> GQTKNEVSQDTIKTFTLPAIPQIMVAPEQRAEFLVKHYWDNVNFADTNYIHHPEITEQAWVDYCDILNHVPLKTAQEAIRKTIDRTNVDKKVFAYITDLADKYLYDPNSPMRNEEFYIPVLEAMAA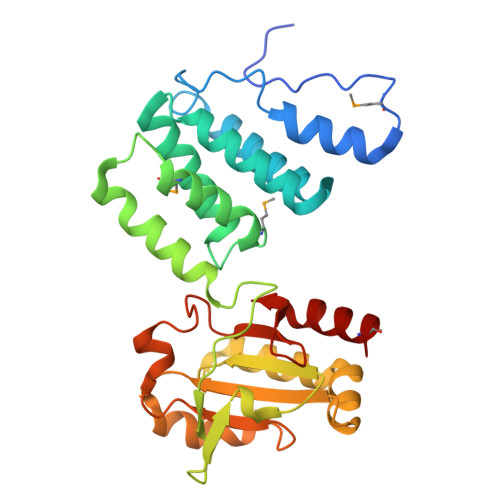SPVLEEIEKVRPKARLELAQKNRIGTKAINFTYTLASGAQGSLYQLNADYLLLFINNPGCHACTETIEGLKQAPIISQLIKEKKLIVLSIYPDEELDDWRKHLNEFPKEWINGYDKKFTIKEKQLYDLKAIPTLYLLNKEKTVLLKDATTQAIEEYLMIHQ>[4x]GMSGIKSLELLLQSMSPELMAGDYVFCTVNGALSDYLSLEPIATFREPEGLTLVLEAEKAQQAGLESSALFS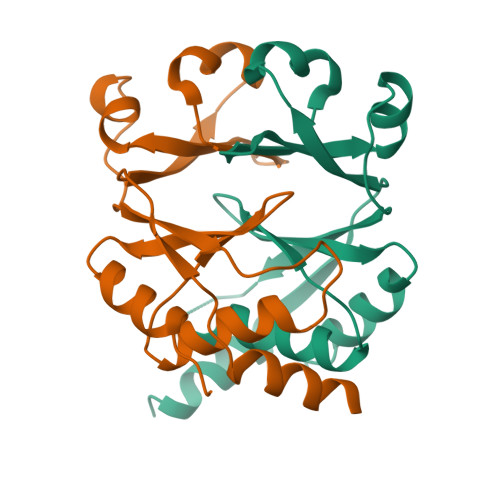LITLTVHSSLEAVGLTAAFATKLAEHGISANVIAGYYHDHIFVQKEKAQQALQALGEFAQA>SLEHHHHHHENLYFQGVGTRWAVLVAGSSGYGNYRHQADVCHAYQILRKGGLKEENIVVLMYDDIANHPLNPRPGTLINHPDGDDVYAGVPKDYTGSSVTAANFYAVLLGDQKAVKGGSGKVIASKPNDHIFVYYANHGGPGVLGMPNTPHIYAADFIETLKKKHASGTYKEMVIYVEAAESGSIFEGIMPKDLNIYVTTASNAQESSYGTYCPGMNPSPPSEYITCLGDLYSVAWMEDSETHNLKKETIKQQYHTVKMRTSNYNTYSGG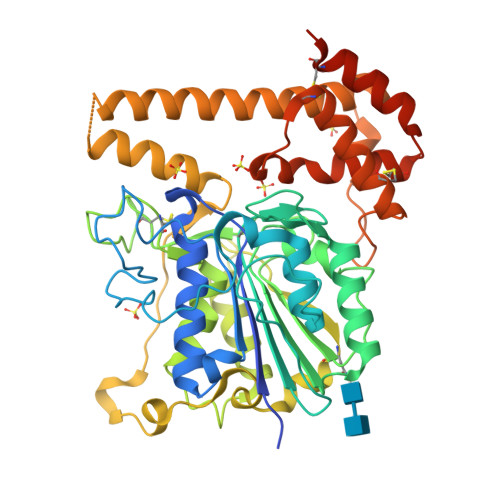SHVMEYGNNSIKSEKLYLYQGFDPATVNLPLNELPVKSKIGVVNQRDADLLFLWHMYRTSEDGSRKKDDTLKELTETTRHRKHLDASVELIATILFGPTMNVLNLVREPGLPLVDDWECLKSMVRVFEEHCGSLTQYGMKHMRAFANVCNNGVSKELMEEASTAACGGYSEARYTVHPSILGYSA[12x]> MHHHHHHMRGSMASEIHMTGPMCLIENTNGRLMANPEALKILSAITQPMVVVAIVGLYRTGKSYLMNKLAGKKKGFSLGSTVQSHTKGIWMWCVPHPKKPGHILVLLDTEGLGDVEKGDNQNDSWIFALAVLLSSTFVYNSIGTINQQAMDQLYYVTELTHR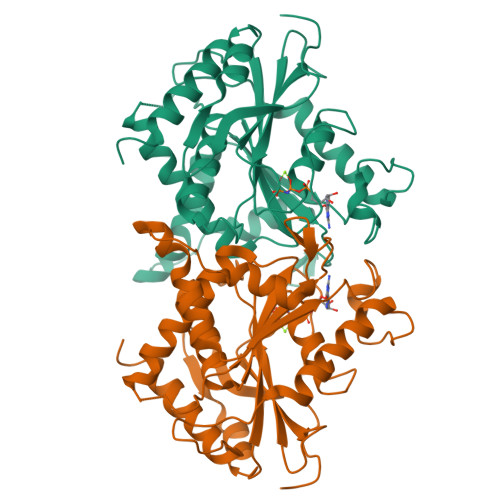IRSKSSPDENENEVEDSADFVSFFPDFVWTLRDFSLDLEADGQPLTPDEYLTYSLKLKKGTSQKDETFNLPRLCIRKFFPKKKCFVFDRPVHRRKLAQLEKLQDEELDPEFVQQVADFCSYIFSNSKTKTLSGGIQVNGPRLESLVLTYVNAISSGDLPCMENAVL> MEPLLLAWSYFRRRRFQLCADLCTQMLEKSPCDQAAWILKARALTEMVYVDEIDVDEEGIAEMILDENAIAQVPRPGTSLKLPGTNQTGGPSPAVRPVTQAGRPITGFLRPSTQSGRPGTIEQAIKTPRTAYTARPIASSSGRFVRLGTASMLTSPDGPFINLSRLNLAKYAQKPKLAKALFEYIFHHENDVKTALDLAALSTEHSQYKDWWWKVQIGKCYYRLGLYREAEKQFKSALKQQEMVDTFLYLAKVYISLDQPLTALNLFKQGLDKFPGEVTLLCGIARIYEEMNNISSATEYYKEVLKQDNTHVEAIACIGSNHFYTDQPEVALRFYRRLLQMGVYNCQLFNNLGLCCFYAQQYDMTLTSFERALSLAENEEEVADVWYNLGHVAVGTGDTNLAHQCFRLALVSNNQHAEAYNNLAVLEMRRGHVEQAKALLQTASSLAPHMYEPHFNFATISDKIGDLQRSYAAAKKSEAAFPDHVDTQHL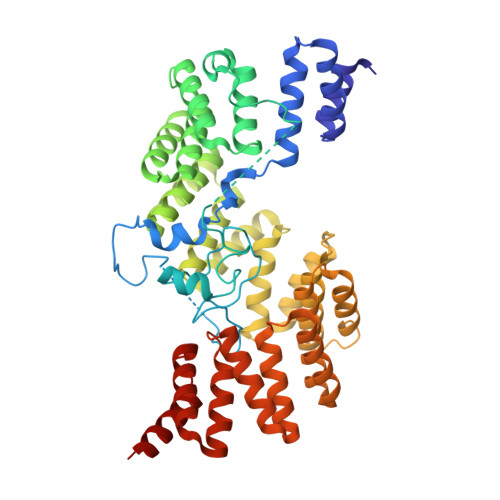IKQLEQHFAML> GGTGGGGCAGGCCCCACC

Nine new crystal structures of CG-rich DNA 18-mers with the sequence 5′-GGTGGGGGC-XZ-GCCCCACC-3′, which are related to the bacterial repetitive extragenic palindromes, are reported. All 18-mers crystallized as isomorphic tetragonal crystals with one strand of a right-handed antiparallel duplex in the asymmetric unit. All reported structures co-crystallized with the Sr2+ cation located between nucleotides 6 and 7 and (by symmetry) 12 and 13.

Finally, only one of the four RR variants, Chom-18-AG, was crystallized. The crystals of Chom-18-AG diffracted to the lowest crystallographic resolution of ∼3 Å. The refinement was initially unstable, producing several negative peaks along the sugar-phosphate backbone in the map and unsatisfactory R work and R free values of 0.305 and 0.431, respectively. To improve the results of refinement, we generated the NtC restraints, which provided torsional refinement parameters for phenix.refine. This decreased the R work and R free values to final values of 0.297 and 0.322, respectively. In addition to this improvement, we also noticed cleaner electron-density maps with fewer diffraction minima along the sugar-phosphate backbone compared with the starting phases of the refinement cycle. The average confal score (the confal score quantifies the agreement between the analyzed dinucleotides and the NtC-defining conformers; for details, see Schneider et al., 2018) for the entire structure increased significantly from 46 to 64, corresponding to a shift from the 47th to the 84th percentile with respect to all nucleic acid structures in the PDB. The A–G pair is strongly nonplanar; despite this, the pair is classified. Most dinucleotides with deformed backbones and unassigned dinucleotides are observed in Chom-18-YY and especially Chom-18-AG, pointing to a highly deformed backbone. The poor quality of the Chom-18-AG crystals and the unsuccessful crystallization of the three R–R 18-mers with central GG, GA and AA dinucleotides may indicate that the central pairs of these R–R 18-mers are becoming too large to be accommodated in the same helical architecture.>[2x]GSHMMERPQPDSMP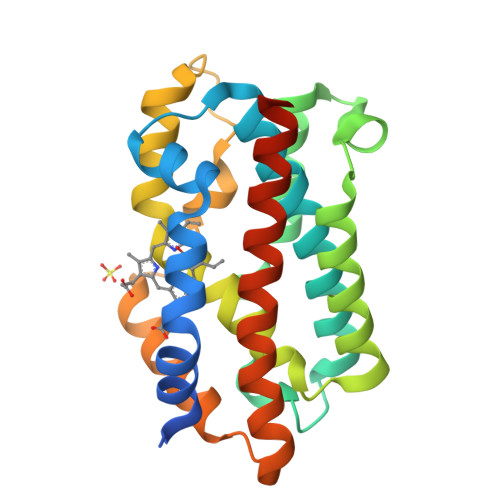QDLSEALKEATKEVRTQAENAEFMRNFQKGQVTRDGFKLVMASLYHIYVALEEEIERNKESPVFAPVYFPEELHRKAALEQDLAFWYGPRWQEVIPYTPAMQRYVKRLHEVGRTEPELLVAHAYTRYLGDLSGGQVLKKIAQKALDLPSSGEGLAFFTFPNIASATKFKQLYRSRMNSLEMTPAVRQRVIEEAKTAFLLNIQLFEELQELLTHDTKDQSPSRA>GHMAPL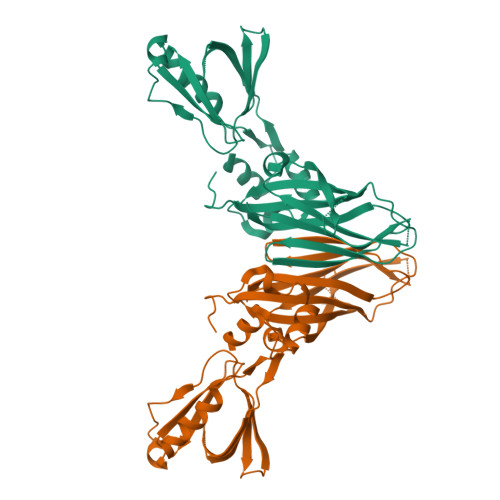PLGRFYIHLNSILNISISEVHSPIKIIVNTPTQNMQLPWQAVNGNNRLDHDFAFHVDDNFKVSFMFLDIPIEDKSNGSKGVSATKDVSNGKPAETKSKAGGSTGSSGGSVVIKKVSGTATLNLGNVKDSCFGKAFNVEIPIISRGFLEAIPVKINSIGKRTLGNLTLTCLYIPELSVPEQELPFTLEQATMDLRHVRSNYLYNEGYLYRLEDSSIRRRFVVLRSKQLNFYAEKGGQYLDTFQLSKTVVSIPMVNFSEAVSNLGLVAGILATSVDRRHVQLFADSKKVCQKWLQVMNSRSFALDRGTEKLWLQEYVNFMA[3x]>RTIVVTTILESPYVMYKKNHEQLEGNERYEGYCVDLAYEIAKHVRIKYKLSIVGDGKYGARDPETKIWNGMVGELVYGRADIAVAPLTITLVREEVIDFSKPFMSLGISIMIKKGTPIESAEDLAKQTEIAYGTLASGSTKEFFRRSKIAVYEKMWSYMKSAEPSVFTKTTADGVARVRKSKGKFAFLLESTMNEYIEQRKPCDTMKVGGNLDSKGYGVATPKGSALGNAVN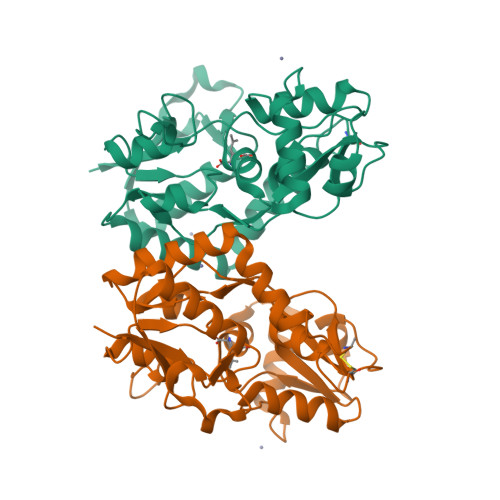LAVLKLNEQGLLDKLKNKWWYDKGEC[2x]1-methyl-~{N}-[2-[[(2~{S})-2-methylpyrrolidin-1-yl]methyl]-3~{H}-benzimidazol-5-yl]indazole-5-carboxamide | C22 H24 N6 O | 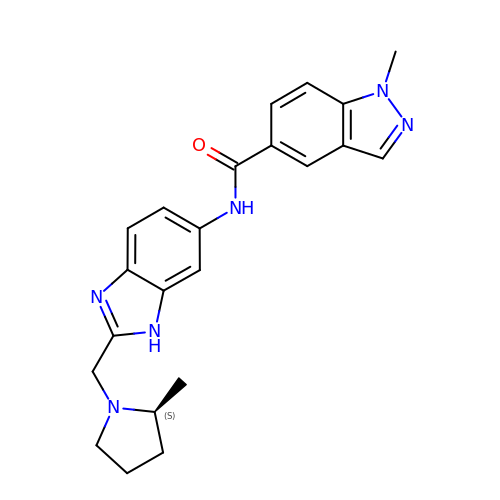QGNDVASWIHEXCL-AWEZNQCLSA-N> MITTPLVHVASVEKGRSYEDFQKVYNAIALK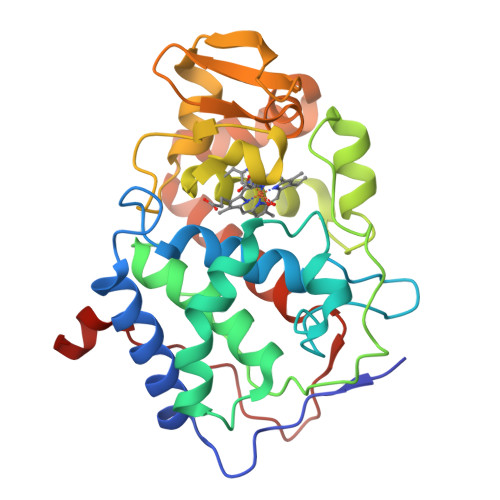LREDDEYDNYIGYGPVLVRLAWHISGTWDKHDNTGGSYGGTYRFKKEFNDPSNAGLQNGFKFLEPIHKEFPWISSGDLFSLGGVTAVQEMQGPKIPWRCGRVDTPEDTTPDNGRLPDADKDAGYVRTFFQRLNMNDREVVALMGAHALGKTHLKNSGYEGPFGAANNVFTNEFYLNLLNEDWKLEKNDANNEQWDSKSGYMMLPTDYSLIQDPKYLSIVKEYANDQDKFFKDFSKAFEKLLENGITFPKDAPSPFIFKTLEEQGL> MTVYNATFTINFYNEGEWGGPEPYGYIKAYLTNPDHDFE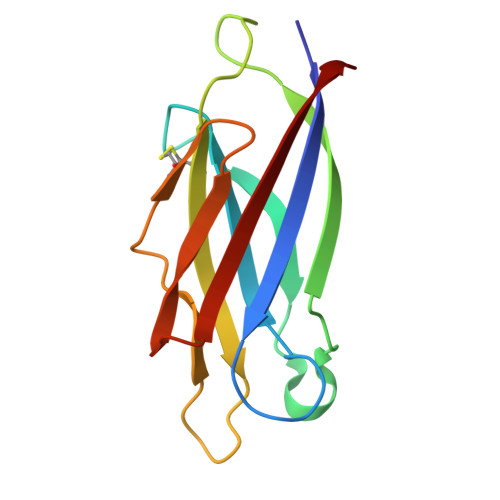IWKQDDWGKSTPERSTYTQTIKISSDTGSPINQMCFYGDVKEYDVGNADDILAYPSQKVCSTPGVTVRLDGDEKGSYVTIKYSLTPA> ELGDSLEEFLAKATTDKNLARLLVCMGEALRTIAFKVRTASCGATACVNTFGDEQLAVDMLADKLLFE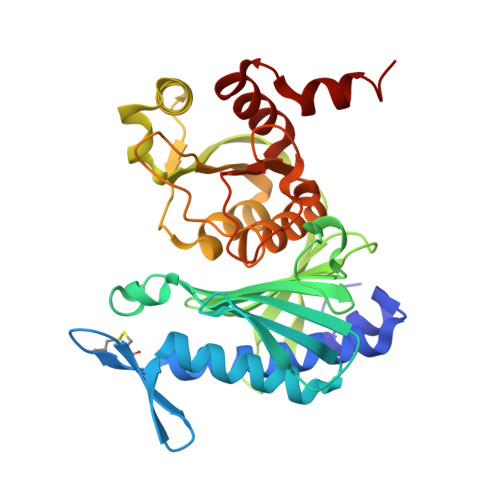ALRHSHVCKYACSEEEPILQDMEGEGFSVAFDPLDGSSIVDTNFTVGTIFGVWPGDKLTGITGRDQAASAMGIYGPRTTYVVAINGFPGTHEFLLMDDGKWQHVKETTEIKEGKLFSPGNLRATFDNADYEKLINYYVSEKYTLRYTGGMVPDVNQIIVKERGIFTNVTSPTTKAKLRLLFEVAPLGLLIENAGGYSSDGKQSVLDKVVVNTDDRTQVAYGSRDEIIRFEETLYGDSRLKAELAAATV> SPVEWTVMDVVEYFTEAGFPEQATAFQEQEIDGKSLLRMQRTDVLTGLSIRLGPALKIYEHHIKVL;> GSVSKWST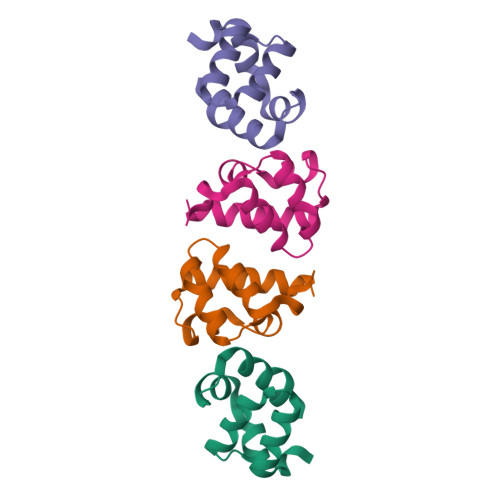DEVSEFIQSLPGCEEHGKVFKDEQIDGEAFLLMTQTDIVKIMSIKEGPAEKIFNSILMFKAAEKN>DVSGTVCLSALPPEATDTLNLIASD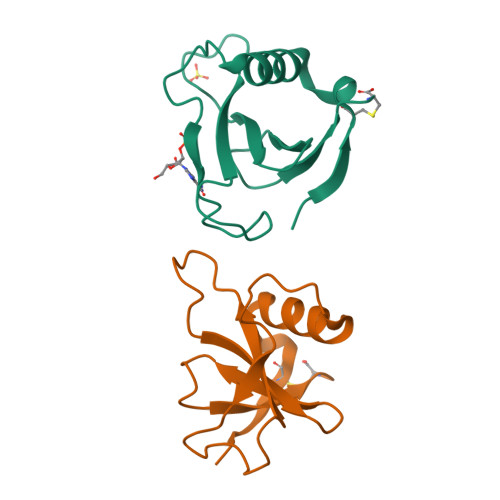GPFPYSQDGVVFQNRESVLPTQSYGYYHEYTVITPGARTRGTRRIITGEATQEDYYTGDHYATFSLIDQTC[2x]> GPMPFYDSRPPEGWPKGSINDMDYPLLGSICAVCCVFVAGSGIWMLYRLDLGMGYSCKPYKSGRAPEVNSLSGIICLLCGTMYAAKSFDFFDGGGTPFSLNWYWYLDYVFTCPLLILDFAFTLDLPHKIRYFFAVFLTLWCGVAAFVTPSAYRFAYYALGCCWFTPFALSLMRHVKERYLVYPPKCQRWLFWACVIFFGFWPMFPILFIFSWLGTGHISQQAFYIIHAFLDLTCKSIFGILMTVFRLELEEHTEVQGLPLNEPETLSLEVLFQ

KCR channelrhodopsins (K+-selective light-gated ion channels) have received attention as potential inhibitory optogenetic tools but more broadly pose a fundamental mystery regarding how their K+ selectivity is achieved. Here, we present 2.5–2.7 Å cryo-electron microscopy structures of HcKCR1 and HcKCR2 and of a structure-guided mutant with enhanced K+ selectivity. Structural, electrophysiological, computational, spectroscopic, and biochemical analyses reveal a distinctive mechanism for K+ selectivity; rather than forming the symmetrical filter of canonical K+ channels achieving both selectivity and dehydration, instead, three extracellular-vestibule residues within each monomer form a flexible asymmetric selectivity gate, while a distinct dehydration pathway extends intracellularly.

We expressed HcKCR1 and HcKCR2 in Sf9 insect cells and reconstituted purified proteins into lipid nanodiscs (STAR Methods); cryo-EM structures in the dark state were resolved at 2.6 and 2.5 Å, respectively. The high-resolution density maps allowed accurate modeling of most residues of both HcKCRs (residues 6–260 for HcKCR1 and 2–260 for HcKCR2), as well as water molecules, lipids, and all-trans-retinal with conformer also validated by high-performance liquid chromatography (HPLC). The monomers exhibit an extracellular N-terminal region (residues 6–21 for HcKCR1 and 2–21 for HcKCR2), an intracellular C-terminal region (residues 255–260 for both), and 7 TM domains (within residues 22–254 for both), connected by three intracellular loops (ICL1–3) and three extra-cellular loops (ECL1–3). However, we noted three key differences in HcKCRs: (1) K84 points toward the extracellular side, (2) no water molecules are observed between the Schiff base proton and the two aspartates (D105 and D229), and (3) the highly conserved arginine on ECL1 (R112 in ChRmine) is replaced by a tryptophan (W102 in HcKCRs). We found that the ion passes between N99, W102, and Y222, which we refer to as the selectivity triad, and then enters the extracellular vestibule with minimal protein distortion. As the K+ ion passes through the triad, it forms a π-cation interaction with W102 and polar interactions with the carbonyl group of N99 and the hydroxyl group of Y222; at this stage. the K+ ion is largely dehydrated with just two coordinated water molecules. In WT HcKCR1, we noticed that the selectivity triad stochastically deviated from the cryo-EM conformation, adopting a more open structure with Y222 rotating away from W102. We refer to the Y222 conformation similar to that of the cryo-EM structure as conformation 1 (tight) and the Y222 conformation positioned farther from W102 as conformation 2 (loose). WT simulations suggested that when Y222 adopts the loose conformation, the triad architecture becomes significantly opened, transiently reducing channel selectivity.>[2x]SDSLSK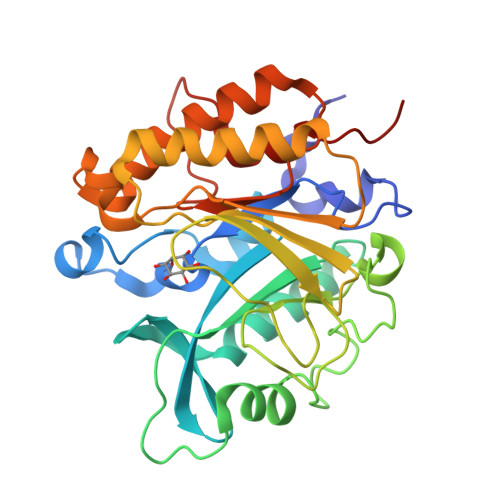SPENWMSKLDDGKHLTEINIPGSHDSGSFTLKDPVKSVWAKTQDKDYLTQMKSGVRFFDIRGRASADNMISVHHGMVYLHHELGKFLDDAKYYLSAYPNETIVMSMKKDYDSDSKVTKTFEEIFREYYYNNPQYQNLFYTGSNANPTLKETKGKIVLFNRMGGTYIKSGYGADTSGIQWADNATFETKINNGSLNLKVQDEYKDYYDKKVEAVKNLLAKAKTDSNKDNVYVNFLSVASGGSAFNSTYNYASHINPEIAKTIKANGKARTGWLIVDYAGYTWPGYDDIVSEIIDSNKLEHHHHHH>MSGTEEAILGGRDSHPAAGGGSVLCFGQCQYTAEEYQAIQKALRQRLGPEYISSRMAGGGQKVCYIEGHRVINLANEMFGYNGWAHSITQQNVDFVDLNNGKFYVGVCAFVRVQLKDGSYHEDVGYGVSEGLKSKALSLEKARKEAVTDGLKRALRSFGNALGNCILDKDYLRSLNKLPRQLPLEVDLTKAKRQDLEPSVEEARYNSCRPNMALGHPQLQQVTSPSRPSHAVIPADQDCSSRSLSSSAVESEATHQRKLRQKQLQQQFRERMEKQQVRVSTPSAEKSEAAPPAPPVTHSTPVTVSEPLLEKDFLAGVTQELIKTLEDNSEKWAVTPDAGDGVVKPSSRADPAQTSDTLALNNQMVTQNRTPHSVCHQ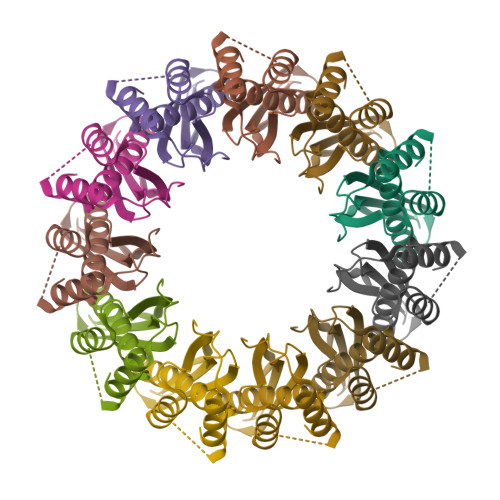KPQAKSGSWDLQTYSADQRTTGNWESHRKSQDMKKRKYDPS[11x]> KKATATTT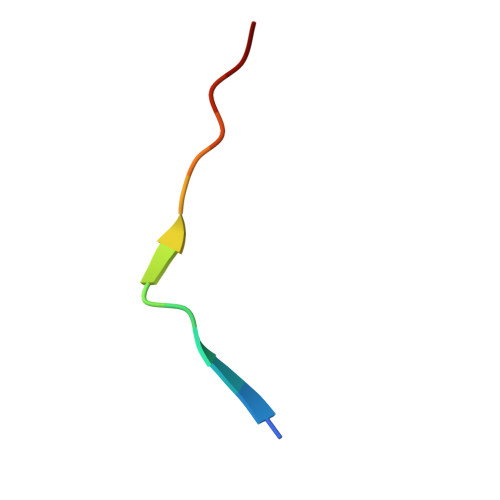WMVPTA>[2x]NTALAEMPKRKFTIDDFDIGRPLGKGKFGNVYLAREKQNKFIMALKVLFKSQLEKEGVEHQLRREIEIQSHLRHPNILR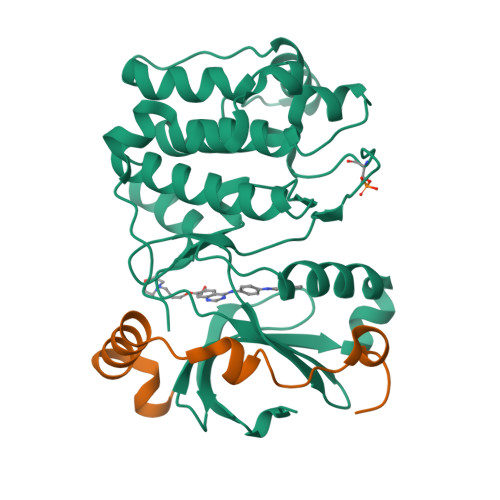MYNYFHDRKRIYLMLEFAPRGELYKELQKHGRFDEQRSATFMEELADALHYCHERKVIHRDIKPENLLMGYKGELKIADFGWSVHAPSLRRRTMCGTLDYLPPEMIEGKTHDEKVDLWCAGVLCYEFLVGMPPFDSPSHTETHRRIVNVDLKFPPFLSDGSKDLISKLLRYHPPQRLPLKGVMEHPWVKANSRRVLPPVYQSTQSK;>[2x]IPAWASGNLLTQAIRQQYYKPIDVDRMYGTIDSPKLEELFNKS> SNAMDFNELFPVGTYRRMVKKVSVSDTVTNRSKALEEFMSTAAFLETMTQLAVEILDHKLPEGFVSVGVRSEVHNLAPAVLGDDVTFTVTVDRVEGNRVVLSMKADDPHGPVATGLQERVVVSTDLLEKRVWER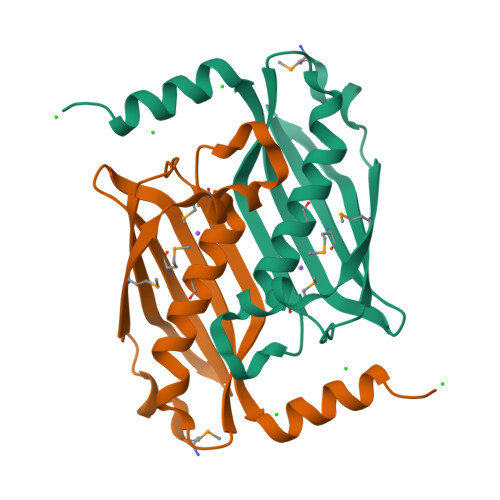FGGR> GPQSEPELKLESVVIVSRHGVRAPTKATQLMQDVTPDAWPTWPVKLGWLTPRGGELIAYLGHYQRQRLVADGLLAKKGCPQSGQVAIIADVDERTRKTGEAFAAGLAPDCAITVHTQADTSSPDPLFNPLKTGVCQLDNANVTDAILSRAGGSIADFTGHRQTAFRELERVLNFPQSNLCLKREKQDESCSLTQALPSELKVSADNVSLTGAVSLASMLTEIFLLQQAQGMPEPGWGRITDSHQWNTLLSLHNAQFYLLQRTPEVARSRATPLLDLIKTALTPHPPQKQAYGVTLP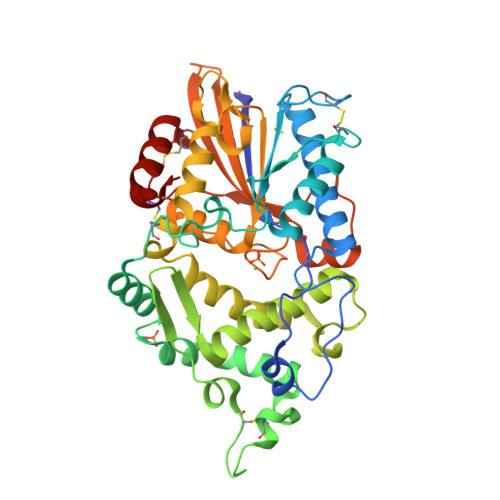TSVLFIAGHDTNLANLGGALELNWTLPGQPDNTPPGGELVFERWRRLSDNSQWIQVSLVFQTLQQMRDKTPLSLNTPPGEVKLTLAGCEERNAQGMCSLAGFTQIVNEARIPACSL>GCSTPLGMENGKIENKQITASSFKKSWWGDYWEPFRARLNAQGRVNAWQAKANNNKQWLEIDLLKIKKITAIITQGCKSLSSEMYVKSYTIHYSEQGVEWKPYRLKSSMVDKIFEGNTNTKGHVKNFFNPPIISRFIRVIPKTWNQSITLRLELFGC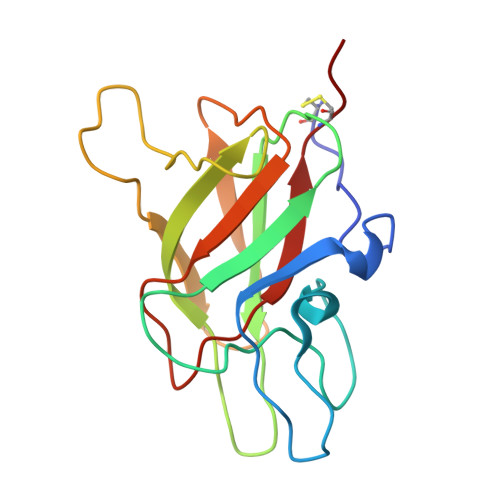DIY[2x]> NAL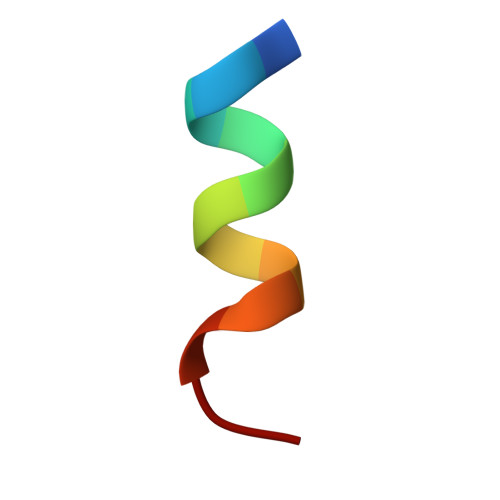LRYLLDRDD> GSKDRTQELRTAKDSDDDDDVTVTVDRDRFMDEFFEQVEEIRGFIDKIAENVEEVKRKHSAILASPNPDEKTKEELEELMSDIKKTANKVRSKLKSIEQSIEQEEGL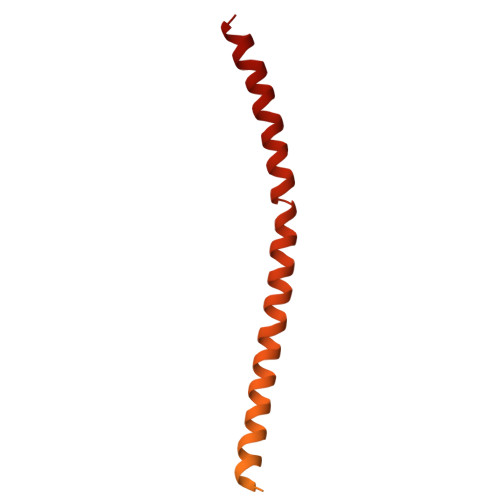NRSSADLRIRKTQHSTLSRKFVEVMSEYNATQSDYRERCKGRIQRQLEITGRTTTSEELEDMLESGNPAIFASGIIMDSSISKQALSEIETRHSEIIKLENSIRELHDMFMDMAMLVESQGEMIDRIEYNVEHAVDYVERAVSDTKK(3beta,5beta,9beta)-3-(propanoyloxy)cholan-24-oic acid | C27 H44 O4 | 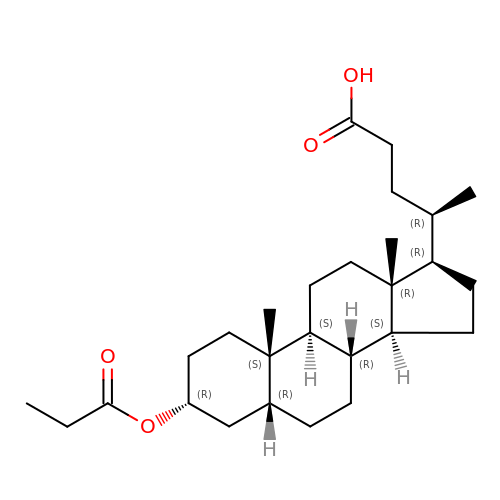RDIKLWFVJHJCMN-RMXYKXGFSA-N>[4x]MSHHHHHHSMDIEFMRILHTSDWHLGQNFYSKSREAEHQAFLDWLLETAQTHQVDAIIVAGDVFDTGSPPSYARTLYNRFVVNLQQTGCHLVVLAGNHDSVATLNESRDIMAFLNTTVVASAGHAPQILPRRDGTPGAVLCPIPFLRPRDIITSQAGLN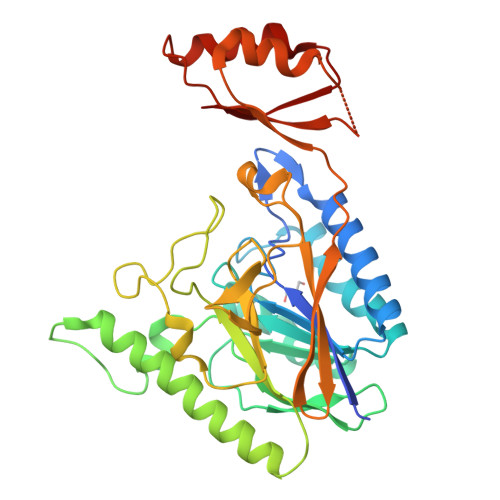GIEKQQHLLAAITDYYQQHYADACKLRGDQPLPIIATGHLTTVGASKSDAVRDIYIGTLDAFPAQNFPPADYIALGHIHRAQIIGGMEHVRYCGSPIPLSFDECGKSKYVHLVTFSNGKLESVENLNVPVTQPMAVLKGDLASITAQLEQWRDVSQEPPVWLDIEITTDEYLHDIQRKIQALTESLPVEVLLVRR(4R)-4-(4-chlorophenoxy)-1-[(4-chlorophenyl)sulfonyl]-N-hydroxy-L-prolinamide | C17 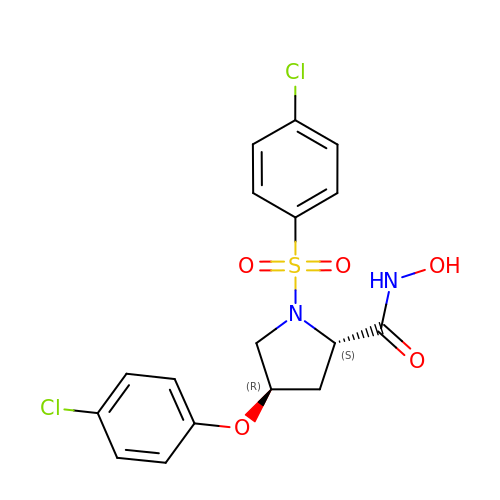H16 Cl2 N2 O5 S | WCAWLFZGKDGOEI-ZBFHGGJFSA-N> SNARPQGLHLELETRLQKMYGIRQVIVVEATEPDDEESIKQAIGSAAAHYLETSLSAQDHIGISSWSS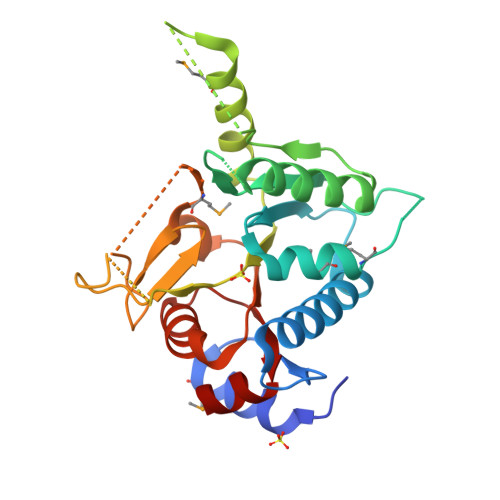TIRAMVSHMHPQPGKQSAQEVVQLLGGVGNKGAFEATLLTQRLATLLNCPAFLLPSQSIEQSVESKQRIVEMEEVKEVLHRFDSITLAIVGIGELEPSQLLRNSGNYYTEDMLRVLAERGAVGDICLRYFDAQGKPVLEEDEEFVVSMGLGKLRSINRVLGLAGGVRKVQAIKGALLGGYLDVLITDVGTARGLGG> MHHHHHHMIEWIIRRSVANRFLVLMGALFLSIWGTWTIINTPVDALPDLSDVQVIIKTSYPGQAPQIVENQVTYPLTTTMLSVPGAKTVRGFSQFGDSYVYVIFEDGTDPYWARSRVLEYLNQVQGKLPAGVSAELGPDATGVGWIYEYALVDRSGKHDLADLRSLQDWFLKYELKTIPDVAEVASVGGVVKEYQVVIDPQRLAQYGISLAEVKSALDASNQEAGGSSIELAEAEYMVRASGYLQTLDDFNHIVLKASENGVPVYLRDVAKVQIGPEMRRGIAELNGEGEVAGGVVILRSGKNAREVIAAVKDKLETLKSSLPEGVEIVTTYDRSQLIDRAIDNLSGKLLEEFIVVAVVCALFLWHVRSALVAIISLPLGLCIAFIVMHFQGLNANIMSLGGIAIAVGAMVDAAIVMIENAHKRLEEWQHQHPDATLDNKTRWQVITDASVEVGPALFISLLIITLSFIPIFTLEGQEGRLFGPLAFTKTYAMAGAALLAIVVIPILMGYWIRGKIPPESSNPLNRFLIRVYHPLLLKVLHWPKTTLLVAALSVLTVLWPLNKVGGEFLPQINEGDLLYMPSTLPGISAAEAASMLQKTDKLIMSVPEVARVFGKTGKAETATDSAPLEMVETTIQLKPQEQWRPGMTMDKIIEELDNTVRLPGLANLWVPPIRNRIDMLSTGIKSPIGIKVSGTVLADIDAMAEQIEEVARTVPGVASALAFRLEGGRYINVEINREKAARYGMTVADVQLFVTSAVGGAMVGETVEGIARYPINLRYPQSWRDSPQALRQLPILTPMKQQITLADVADIKVSTGPSMLKTENARPTSWIYIDARDRDMVSVVHDLQKAIAEKVQLKPGTSVAFSGQFELLERANHKLKLMVPMTLMIIFVLLYLAFRRVGEALLIISSVPFALVGGIWLLWWMGFHLSVATGTGFIALAGVAAEFGVVMLMYLRHAIEAVPSLNNPQTFSEQKLDEALYHGAVLRVRPKAMTVAVIIAGLLPILWGTGAGSEVMSRIAAPMIGGMITAPLLSLFIIPAAYKLMWLHRHRVRK;>MKKIALIIGSMIAGGIISAAGFTWVAKAEPPAEKTSTAERKILFWYDPMYPNTRFDKPGKSPFMDMDLVPKYADEESSASGVRIDPTQTQNLGVKT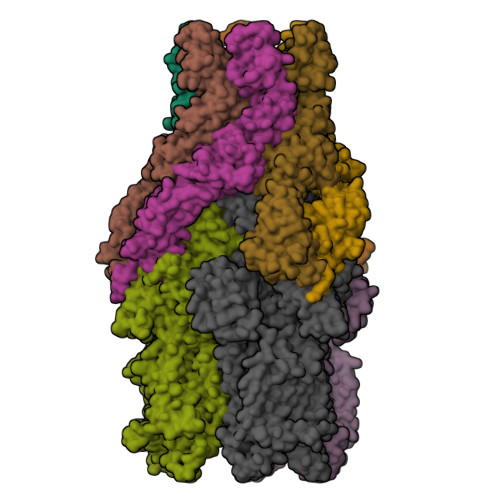ATVTRGPLTFAQSFPANVSYNEYQYAIVQARAAGFIDKVYPLTVGDKVQKGTPLLDLTIPDWVEAQSEYLLLRETGGTATQTEGILERLRLAGMPEADIRRLIATQKIQTRFTLKAPIDGVITAFDLRAGMNIAKDNVVAKIQGMDPVWVTAAIPESIAWLVKDASQFTLTVPARPDKTLTIRKWTLLPGVDAATRTLQLRLEVDNADEALKPGMNAWLQLNTASEPMLLIPSQALIDTGSEQRVITVDADGRFVPKRVAVFQASQGVTALRSGLAEGEKVVSSGLFLIDSEANISGALERMRSESATHAHHHHHHH[2x]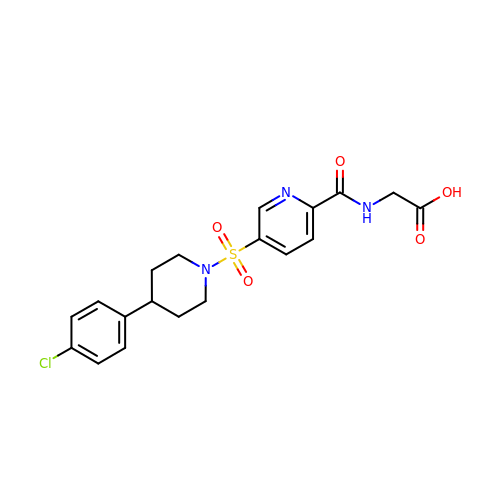N-{5-[4-(4-chlorophenyl)piperidine-1-sulfonyl]pyridine-2-carbonyl}glycine | C19 H20 Cl N3 O5 S | HIWYRXWPCQHOSO-UHFFFAOYSA-N>[4x]MATQGVFTLPANTRFGVTAFANSSGTQTVNVLVNNETAATFSGQSTNNAVIGTQVLNSGSSGKVQVQVSVNGRPSDLVSAQVILTNELNFALVGSEDGTDNDYNDAVVVINWPLG;>XKKLLKCLKCLLKX[3x]

Herein we report the first X-ray crystal structures of mixed chirality α-helices in short peptides comprising only natural residues as the example of a stapled bicyclic and a linear membrane disruptive amphiphilic antimicrobial peptide (AMP) containing seven l- and four d-residues, as complexes of fucosylated analogs with the bacterial lectin LecB. The mixed chirality α-helices are superimposable onto the homochiral α-helices and form under similar conditions as shown by CD spectra and MD simulations but non-hemolytic and resistant to proteolysis. To get a direct insight into the structure of AMBP bp65/bp69 and their linear analogs ln65/ln69, we performed several crystallization studies using either the compounds themselves or their racemates to be crystallized as pure compounds, or their fucosylated derivatives of both mirror image peptides as complexes with the P. aeruginosa lectin LecB. While previous reports of similar mixed chirality AMPs concluded on either unordered conformations or helical conformations appearing in a membrane environment based on deconvolution of FTIR spectra, here we reported X-ray crystallographic evidence of short mixed chirality helices consisting of only natural residues existing as helix bundles within the protein environment of a lectin and almost perfectly superimposable with their parent homochiral α-helices. These direct observations unequivocally demonstrate that the α-helical fold with only natural residues can sometimes tolerate multiple stereochemical inversions without significant conformational changes.

For the mixed chirality AMBP bp69, we obtained two crystal structures of lectin LecB complexed with bp71, an analog of the mixed chirality AMBP bp69 with an additional side-chain fucosylated lysine at the C-terminus. The six individual structures of the mixed chirality AMBP featured essentially the same double-stapled amphiphilic α-helix as that observed in the parent homochiral AMBP structures. Remarkably, the ten crystallographically non-equivalent stapled bicyclic α-helices observed in the X-ray structures of the homochiral rac-bp65 and bp70, and the mixed chirality bp71·LecB complex were essentially superimposable, with RMSD < 0.6 Å for the peptide backbones. In the case of bp65, bp71 and Fln65 the peptides were aggregated in bundles of four of more helices via hydrophobic contacts between leucine side chains. A closer analysis of the different X-ray structures showed that the peptides did not make any significant contact with LecB apart from the anchoring fucose residue. By investigating the structure of AMPBs we discovered the mixed chirality sequence bp69 containing seven l- and four d-residues folding into an amphiphilic α-helix within a stapled bicyclic peptide similar to the parent all l-AMBP bp65.>ETSLGGWLLIQQRMDGSLNFNRTWQDYKRGFGSLNDEGEGEFWLGNDYLHLLTQRGSVLRVELEDWAGNEAYAEYHFRVGSEAEGYALQVSSYEGTAGDALIEGSVEEGAEYTSHNNMQFSTFDRDADQWEENCAEVYGGGWWYNNCQAANLNGIYYPGGSYDPRNNSPYEIENG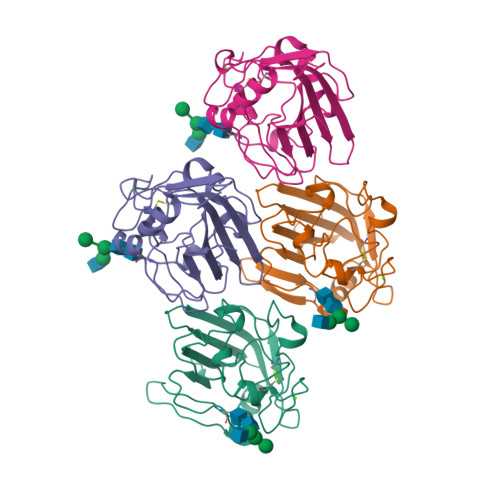VVWVSFRGADYSLRAVRMKIRPLVTQ[8x]>MAKKVAVLAVNPVNGCGLFQYLEAFFENGISYKVFAVSDTKEIKTNSGMVLIVDDVIANLKGHEDEFDALVFSCGDAVPVFQQYANQPYNVDLMEVIKTFGEKGKMMIGHCAGAMMFDFTGITKG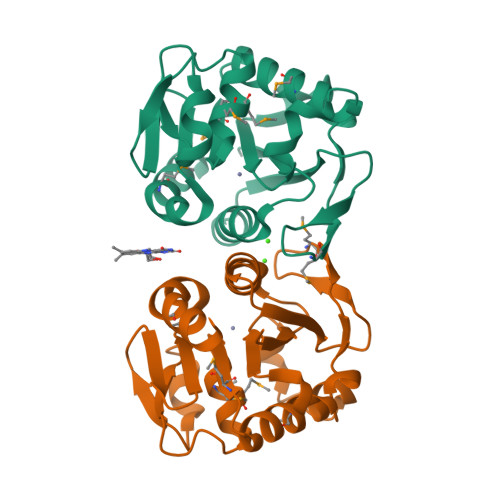KKVAVHPLAKPAIQNGIATDEKSEIDGNFFTAQDENTIWTMLPKVIEALK[4x]> MNWNI;> MAIYADNSYSIGNTPLVRLKHFGHNGNVVVKIEGRNPSYSVKCRIGANMVWQAEKDGTLTKGKEIVDA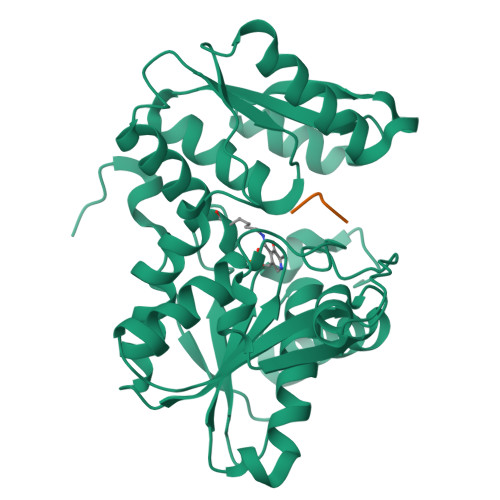TSGNTGIALAYVAAARGYKITLTMPETMSLERKRLLCGLGVNLVLTEGAKGMKGAIAKAEEIVASDPSRYVMLKQFENPANPQIHRETTGPEIWKDTDGKVDVVVAGVGTGGSITGISRAIKLDFGKQITSVAVEPVESPVISQTLAGEEVKPGPHKIQGIGAGFIPKNLDLSIIDRVETVDSDTALATARRLMAEEGILAGISSGAAVAAADRLAKLPEFADKLIVVILPSASERYLSTALFEGIEG> MRCIGISNRDFVEGVSGGSWVDIVLEHGSCVTTMAKNKPTLDFELIKTEAKQPATLRKYCIEAKLTNTTTDSRCPTQGEPSLNEEQDKRFVCKHSMVDRGWGNGCGLFGKGGIVTCAMFTCKKNMKGKVVQPENLEYTIVITPHSGEEHAVGNDTGKHGKEIKITPQSSITEAELTGYGTVTMECSPRTGLDFNEMVLLQMENKAWLVHRQWFLDLPLPWLPGADTQGSNWIQKETLVTFKNPHAKKQDVVVLG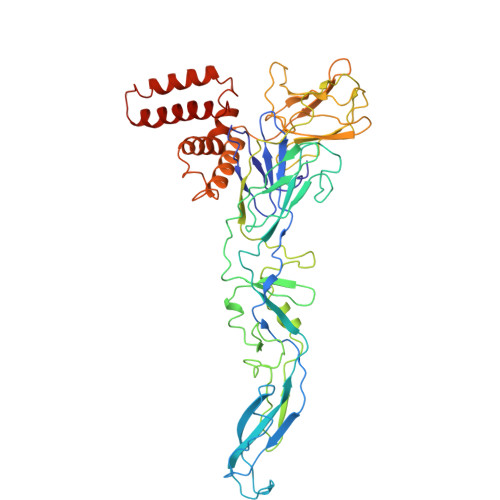SQEGAMHTALTGATEIQMSSGNLLFTGHLKCRLRMDKLQLKGMSYSMCTGKFKVVKEIAETQHGTIVIRVQYEGDGSPCKIPFEIMDLEKRHVLGRLITVNPIVTEKDSPVNIEAEPPFGDSYIIIGVEPGQLKLNWFKKGSSIGQMIETTMRGAKRMAILGDTAWDFGSLGGVFTSIGKALHQVFGAIYGAAFSGVSWIMKILIGVIITWIGMNSRSTSLSVSLVLVGVVTLYLGVMVQA> GASTSEKKTYLETQLDAVMINDQPYTVIFQRAKLKMQDPLELEVLKEVDPCIVRDIDVSEDEVKVVIKPPSSFLTFAAIRKTTLLSRIRAAIHLVSKVKHHSARRLIFIVCPENLMFNRALEPFFLHVGVKESLPPDEWDDERLLREVKATVLALTEGEYRFDEYLKFHETLKCSPIAKELWQADHLDAVLAVLEKWVDEEEAKERAKV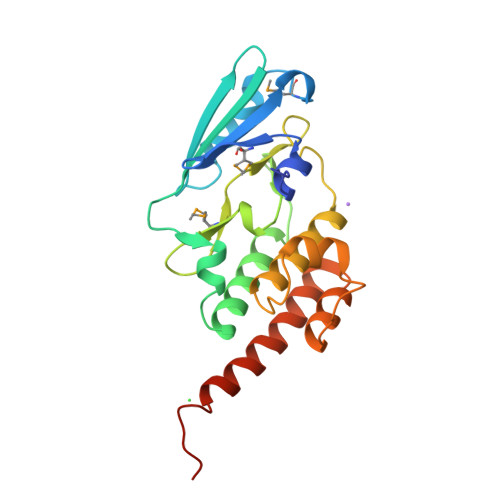HIPKKRWNMQ N-(6-chloropyridin-3-yl)-N~2~-(1,4-dihydro-2H-pyrano[3,4-c]quinolin-9-yl)-L-alaninamide 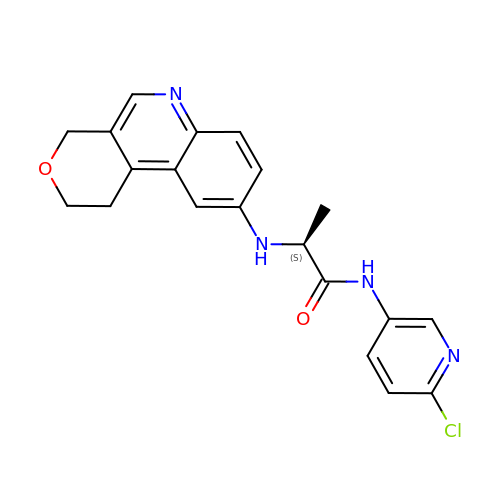| C20 H19 Cl N4 O2 | KABILIUXKOMPNU-LBPRGKRZSA-N(4R,5R)-3-amino-4,5-dihydroxy-cyclohexene-1-carboxylic 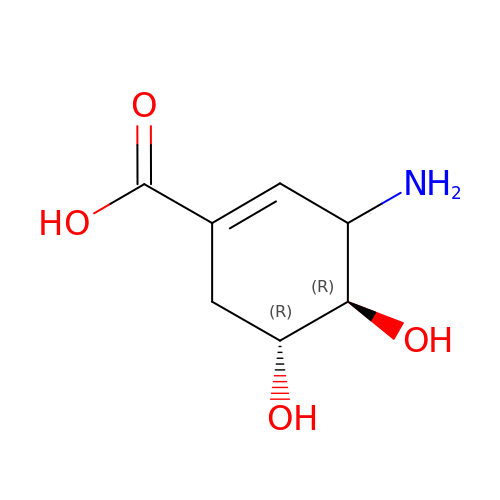acid | C7 H11 N O4 | WPZSUTUAATWRPU-KVQBGUIXSA-N>[4x]MAHHHHHHMANITLKGNAISTVGNLPNIGEQLKDFTLVNADLSEKTLADYKGKK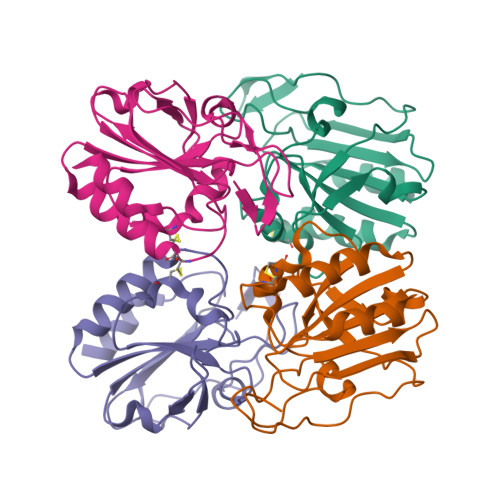VVLNIFPSIDTGVCAASARKFNQEASNLDNTVVVNVSKDLPFALGRFCAAEGLNNVDTLSDFRGHFGDDYGVTLADSPLQGLLSRAVVVADENGNVVYTEQVPEIAQEPNYDAALAALK[[(2~{R},3~{S},4~{R},5~{R})-5-(6-aminopurin-9-yl)-3,4-bis(oxidanyl)oxolan-2-yl]methoxy-oxidanyl-phosphoryl] 2-methyl-2-oxidanyl-propanoate | C14 H20 N5 O9 P | 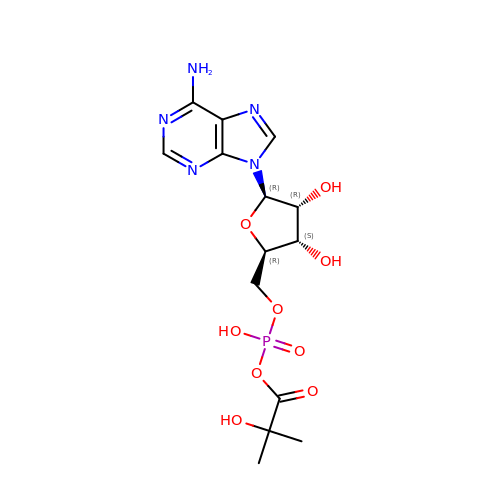WJCYMTFWIDDQPQ-WOUKDFQISA-N>[4x]MDKFRVQGPTRLQGEVTISGAKNAALPILFAALLAEEPVEIQNVPKLKDIDTTMKLLTQLGTKVERDGSVWIDASNVNNFSAPYDLVKTMRASIWALGPLVARFGQGQVSLPGGCAIGARPVDLHIFGLEKLGAEIKLEEGYVKASVNGRLKGAHIVMDKVSVGATVTI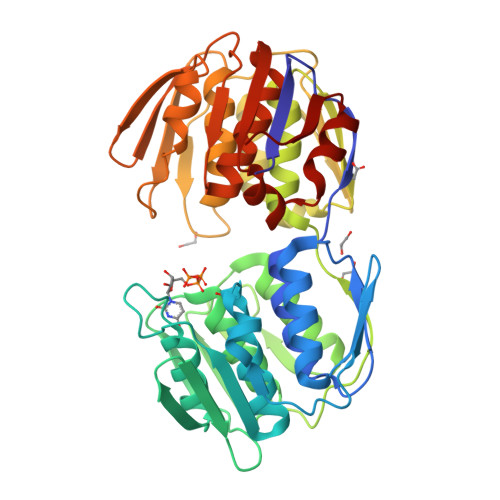MSAATLAEGTTIIENAAREPEIVDTANFLVALGAKISGQGTDRITIEGVERLGGGVYRVLPDRIETGTFLVAAAISGGKIVCRNAQPDTLDAVLAKLREAGADIETGEDWISLDMHGKRPKAVTVRTAPHPAFPTDMQAQFTLLNLVAEGTGVITETIFENRFMHVPELIRMGAHAEIESNTVICHGVEKLSGAQVMATDLRASASLVLAGCIAEGTTVVDRIYHIDRGYERIEDKLRALGANIERVKGE> GGGRHYYWGIPFCPAGVDPNQYTNVILCQLEVYQ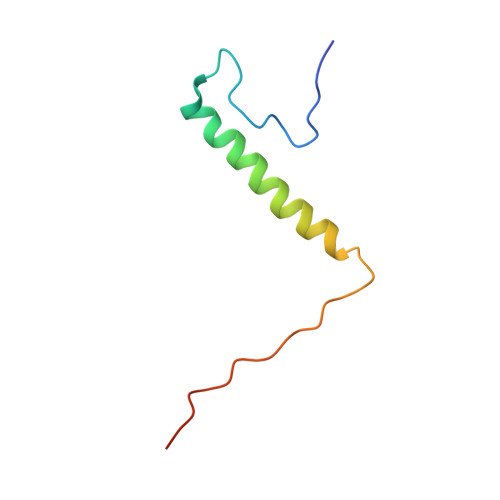KSLKMAQRQLVKKRGFGEPVLPRPPFLIQN3-({(2S)-2-[({(1S)-1-[({(1S)-1-[(R)-CARBOXY(HYDROXY)METHYL]-3,3-DIFLUOROPROPYL}AMINO)CARBONYL]-3-METHYLBUTYL}AMINO)CARBONYL]-2,3-DIHYDRO-1H-INDOL-2-YL}METHYL)THIOPHENE-2-CARBOXYLIC ACID | C26 H31 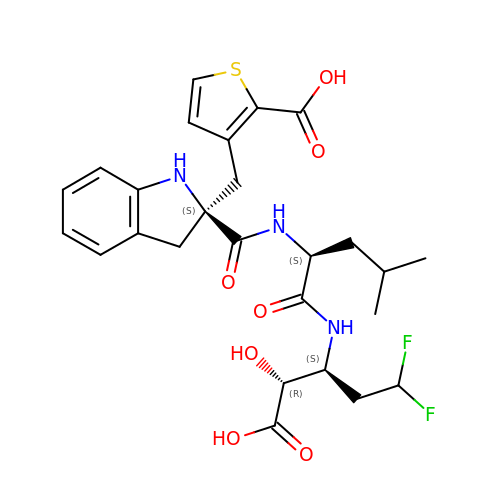F2 N3 O7 S | BEFPIHVRQQQFFB-QUPVEMFASA-N5-{[6-chloro-5-(2'-hydroxy[1,1'-biphenyl]-4-yl)-1H-imidazo[4,5-b]pyridin-2-yl]oxy}-2-methylbenzoic acid | C26 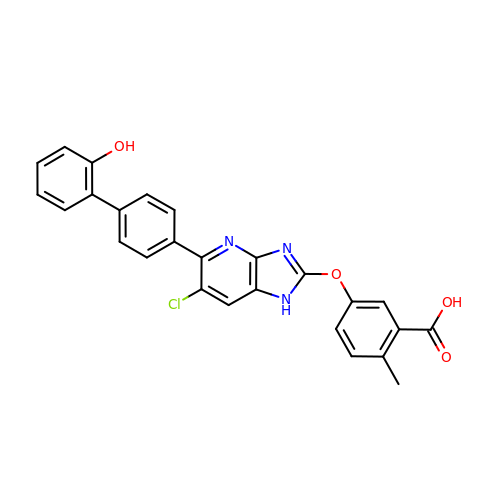H18 Cl N3 O4 | MEZQZPGDJJEQPZ-UHFFFAOYSA-N> CUGG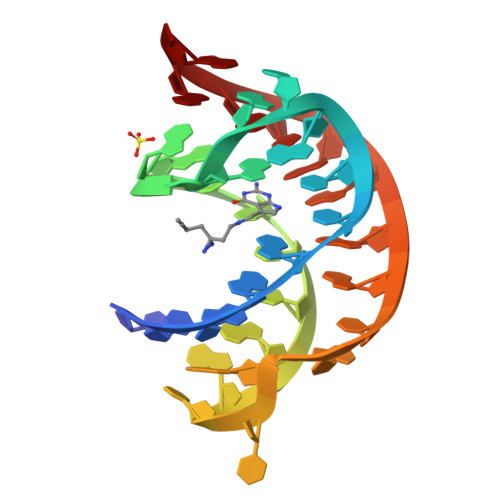GUCGCAGUAACCCCAGUUAACAAAACAAG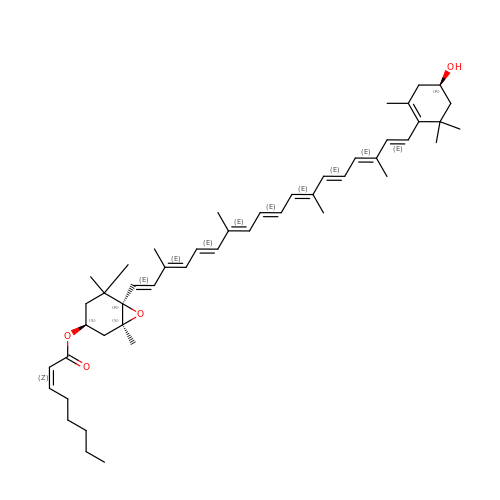[(1~{S},3~{S},6~{R})-1,5,5-trimethyl-6-[(1~{E},3~{E},5~{E},7~{E},9~{E},11~{E},13~{E},15~{E},17~{E})-3,7,12,16-tetramethyl-18-[(4~{R})-2,6,6-trimethyl-4-oxidanyl-cyclohexen-1-yl]octadeca-1,3,5,7,9,11,13,15,17-nonaenyl]-7-oxabicyclo[4.1.0]heptan-3-yl] (~{Z})-oct-2-enoate | C48 H68 O4 | RYRZHZDRYZHUCF-CKQNEJSZSA-N>MAHHHHHHMESLTLQPIARVEGTVNLPGSKSVSNRALLLAALARGTTVLTNLLDSDDVRHMLNALSALGVQYTLSADRTRCEVTGNGGPLRSAAALELFLGNAGTAMRPLAAALCLGSNDIVLTGEPRMKERPIGHLVDALRQGGAQIDCLEQENYPPLRLRGGFQGGNVEVDGSVSSQFLTALLMTAPLAPQDTVIVIKGDLVSKPYIDITLHLMKTFGVEVDNQSYQRFVVRGKQQYQSPGDYLVEGDASSASYFLAAGAIKGGTVKVTGIGRNSVQGDIRFADVLEKMGATVTWGDDFIACTHGELKAVDMDMNHIPDAAMTIATAAL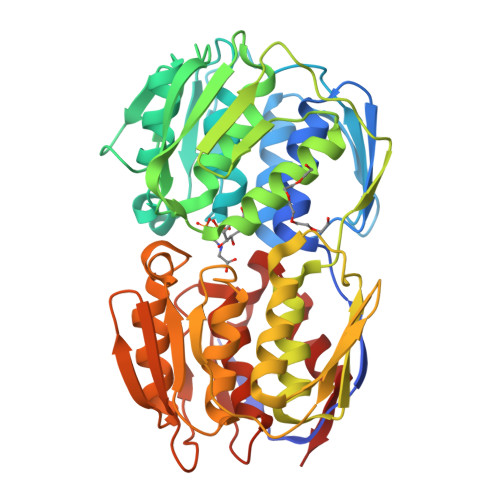FAQGTTTLRNIYNWRVKETDRLFAMATELRKVGAEVEEGEDYIRITPPAKLKYAEIGTYNDHRMAMCFSLVALSDTPVTILDPKCTAKTFPDYFEQLARISTLA[2x]>MGHHHHHHGSGSNRLDGKVAIITGGTLGIGLAIATKFVEEGAAVMITGRHSDVGEKAAKSVGTPDQIQFFQHDSSDEDGWTKLFDATEKAFGPVSTLVNNAGIAVNKSVEETTTAEWRKLLAVNLDGVFFGTRLGIKRMKNKGLGASIINMSSIEGFVGDPSLGAYNASKGAVRIMSKSAALDCALKDYDVRVNTVHPGYIKTPLVDDLPGAEEAMSQRTKTPMGHIGEPNDIAYICVYLASNESKFATGS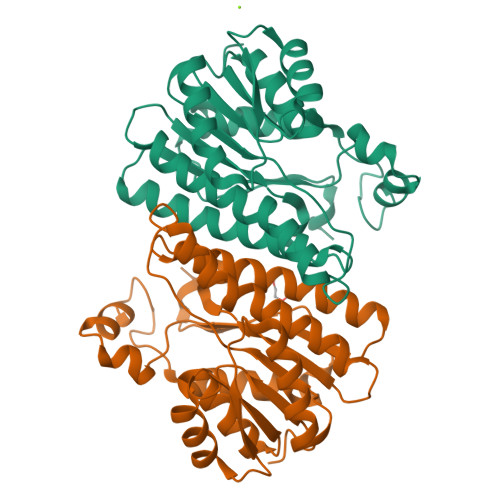EFVVDGGYTAQ[2x]Proliferation and transmission of these obligate endoparasites in their host organisms rely on efficient cell invasion. This active process is based on the motility of the parasite, referred to as gliding, and is empowered by an actin/myosin motor. Actin polymerization occurs between the plasma membrane (PM) and the inner membrane complex (IMC) whereas myosin A is part of the glideosome, which binds the essential light chains ELC and myosin light chain MLC1 (called myosin tail interacting protein, MTIP, in Plasmodium spp.). MLC1 (in P. falciparum: myosin A tail-interacting protein, MTIP) binds at the very C-terminus of MyoA, while ELC is expected to interact with the C-terminus of MyoA upstream of MLC115. We demonstrate that ELCs bind to a conserved binding site on MyoA to induce its α-helical secondary structure and stiffen the MyoA neck.

Heteronuclear NOEs ({1H}-15N NOE) and chemical shift analysis revealed that the protein consists of an α-helical N-terminal domain, while the C-terminal part is disordered. Based on this finding, we were able to determine the structure of the N-terminal PfELC fragment (amino acids 1–74, PfELC-N) by both X-ray crystallography to 1.5 Å resolution and by NMR spectroscopy. The N-terminal domain of PfELC has a typical calmodulin fold with two EF-hands formed by two helix-loop-helix motifs. Both EF-hands lack the canonical residues that usually bind calcium in calmodulins28 and in agreement with that, we did not observe any electron density corresponding to a bound ion. PfELC-N crystallized as a dimer covalently linked via disulfide bridge, but both NMR and non-reducing SDS-PAGE indicate that the protein exists as a monomer in solution and the scattering data calculated from a protein monomer structure fit the measured X-ray scattering profile with Χ2 = 1.37. A comparison between the crystal and the NMR structure highlights that the loop of the first EF hand (residues 16–22) and the third helix (residues 40–47) display the highest degree of flexibility, in agreement with the heteronuclear NOE experiment. The lowest energy NMR conformers are very similar to the crystal structure, with an average backbone RMSD of 1.4 Å over residues 1–68. In general, the assigned backbone resonances in the NMR spectra superimpose for both full-length protein PfELC and the N-terminal domain, proving that the N-terminal domain maintains the same structure as in the full-length context. Contrary to T. gondii TgELCs, the homologous EF hand loop of PfELC (in isolation or in complex) is bent to the other side and does not possess the residues needed for coordination of calcium.

>SMASDMEEKFREAFILFSSCSDHIEMYKFFELMNSFGIILTNDEKAALPNDINMDYWLNFAKKHYNYEQPFKHIN[2x]>[2x]GASMSGEAPRVAVDPFACPMMTMQRKPEVHDAFREAGPVVEVNAPAGGPAWVITDDAL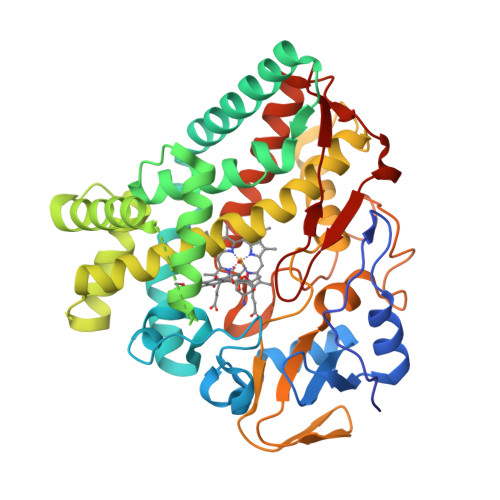AREVLADPRFVKDPDLAPAAWRGVDDGLDIPVPELRPFTLIAVDGEAHRRLRRIHAPAFNPRRLAERTDRIAAIAGRLLTELADASGRSGKPAELIGGFAYHFPLLVICELLGVPVTDPAMAREAVSVLKALGLGGPQSGGGDGTDPAGGVPDTSALESLLLEAVHSARRNDTPTMTRVLYERAQAEFGSVSDDQLVYMITGLIFAGHDTTGSFLGFLLAEVLAGRLAADADEDAVSRFVEEALRYHPPVPYTLWRFAATEVTIGGVRLPRGAPVLVDIEGTNTDGRHHDAPHAFHPDRPSWRRLTFGDGPHYCIGEQLAQLESRTMIGVLRSRFPEARLAVPYDELRWCRKGAQTARLTELPVWLR>TRQFLIYNEDHKRCVDAVSPSAVQTAACNQDAESQKFRWVSESQIMSVAFKLCLGVPSKTDWVAITLYACDSKSEFQKWECKNDTLLGIKGEDLFFNYGNRQEKNIMLYKGSGLWSRWKIYGTTDNLCSRGYEAMYTLLGNANGATCAFPFKFENKWYADCTSAGRSDGWLWCGTTTDYDTDKLFGYCPLKFEGSESLWNKDPLTSVSYQINSKSALTWHQARKSCQQQNAELLSITEIHEQTYLTGLTSSLTSGLWIGLNSLSFNSGWQWSDRSPFRYLNW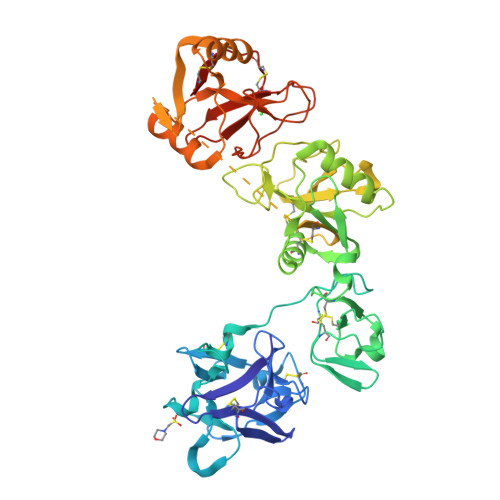LPGSPSAEPGKSCVSLNPGKNAKWENLECVQKLGYICKKGNTTLNSFVIPSESDVPTHCPSQWWPYAGHCYKIHRDEKKIQRDALTTCRKEGGDLTSIHTIEELDFIISQLGYEPNDELWIGLNDIKIQMYFEWSDGTPVTFTKWLRGEPSHENNRQEDCVVMKGKDGYWADRGCEWPLGYICKMKSHHHHHH[8x]> EEFDAIKIALASPDMIRSWSFGEVKKPETINYRTFKPERDGLFCARIFGPVKDYECLCGKYKRLKHRGVICEKCGVEVTQTKVRRERMGHIELASPTAHIWFLKSLPSRIGLLLDMPLRDIERVLYFESYVVIEGGMTNLERQQILTEEQYLDALEEFGDEFDAKMGAEAIQALL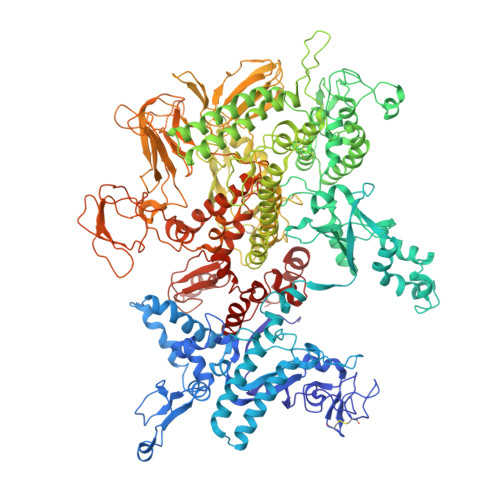KSMDLEQECEQLREELNETNSETKRKKLTKRIKLLEAFVQSGNKPEWMILTVLPVLPPDLRPLVPLDGGRFATSDLNDLYRRVINRNNRLKRLLDLAAPDIIVRNEKRMLQEAVDALLDNGRRGRAITGSNKRPLKSLADMIKGKQGRFRQNLLGKRVDYSGRSVITVGPYLRLHQCGLPKKMALELFKPFIYGKLELRGLATTIKAAKKMVEREEAVVWDILDEVIREHPVLLNRAPTLHRLGIQAFEPVLIEGKAIQLHPLVCAAYNADFDGDQMAVHVPLTLEAQLEARALMMSTNNILSPANGEPIIVPSQDVVLGLYYMTRDCVNAKGMVLTGPAERLYRSGLASLHARVKVRITEYEKDANGELVAKTSLKDTTVGRAILWMIVPKGLPYSIVNQALGKKAISKMLNTCYRILGLKPTVIFADQIMYTGFAYAARSGASVGIDDMVIPEKKHEIISEAEAEVAEIQEQFQSGLVTAGERYNKVIDIWAAANDRVSKAMMDNLQTETVINRDGQEEKQVSFNSIYMMADSGARGSAAQIRQLAGMRGLMAKPDGSIIETPITANFREGLNVLQYFISTHGARKGLADTALKTANSGYLTRRLVDVAQDLVVTEDDCGTHEGIMMTPVIEGGDVKEPLRDRVLGRVTAEDVLKPGTADILVPRNTLLHEQWCDLLEENSVDAVKVRSVVSCDTDFGVCAHCYGRDLARGHIINKGEAIGVIAAQSIGEPGTQLTMRTFHIGGAASRAAAESSIQVKNKGSIKLSNVKSVVNSSGKLVITSRNTELKLIDEFGRTKESYKVPYGAVLAKGDGEQVAGGETVANWDPHTMPVITEVSGFVRFTDMIDGQTITRQTDELTGLSSLVVLDSAERTAGGKDLRPALKIVDAQGNDVLIPGTDMPAQYFLPGKAIVQLEDGVQISSGDTLARIPQESGGTKDITGGLPRVADLFEARRPKEPAILAEISGIVSFGKETKGKRRLVITPVDGSDPYEEMIPKWRQLNVFEGERVERGDVISDGPEAPHDILRLRGVHAVTRYIVNEVQDVYRLQGVKINDKHIEVIVRQMLRKATIVNAGSSDFLEGEQVEYSRVKIANRELEANGKVGATYSRDLLGITKASLATESFISAASFQETTRVLTEAAVAGKRDELRGLKENVIVGRLIPAGTGYAYHQDRMRRRAAG>MKGGNADSWQREKLASMESPEEPGASMDENYFVNYTFKDRSHSGRVAQGIMKLCLEEELFADVTISVEGREFQLHRLVLSAQSCFFRSMFTSNLKEAHNRVIVLQDVSESVFQLLVDYIYHGTVKLRAEELQEIYEVSDMYQLTSLFEECSRFLARTVQVGNCLQVMWLADRHSDPELYTAAKHCAKTHLAQLQNTEEFLHLP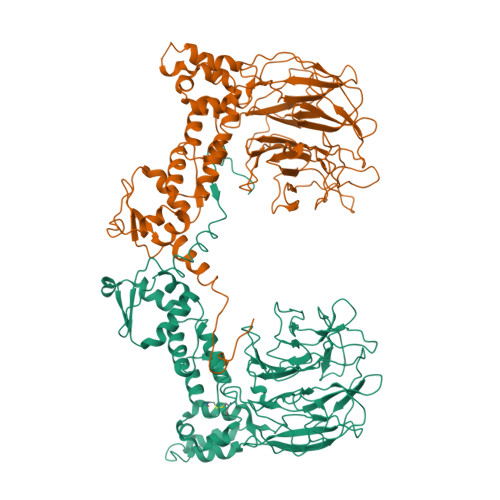HRLLTDIISDGVPCSQNPTEAIEAWINFNKEEREAFAESLRTSLKEIGENVHIYLIGKESSRTHSLAVSLHCAEDDSISVSGQNSLCHQITAACKHGGDLYVVGGSIPRRMWKCNNATVDWEWCAPLPRDRLQHTLVSVPGKDAIYSLGGKTLQDTLSNAVIYYRVGDNVWTETTQLEVAVSGAAGANLNGIIYLLGGEENDLDFFTKPSRLIQCFDTETDKCHVKPYVLPFAGRMHAAVHKDLVFIVAEGDSLVCYNPLLDSFTRLCLPEAWSSAPSLWKIASCNGSIYVFRDRYKKGDANTYKLDPATSAVTVTRGIKVLLTNLQFVLA[2x]>GPGSMTTPNFELYGYFRSSCSGRLRIAFHLKSIPYTRHPVNLLKGEQHSDTYKSLNPTNTVPLLVVSNINNTVSPSSASFSIGQSLAALEYLEEALPTNARPLLPPISNPVARAHVRTICNIIACDVQPVTNLKIQKKVKALDGDPTVWSRDLATQGFGAVEKLLELSAGRFCVGDEITLADVCLVPAVWAAERVGMDLARFPITKRVFEEMLKEEAVQKAHWQKQEDTPEDLRA[4x]

Crystal structures are presented for a putative uncharacterized protein that shares sequence similarity with ζ-class glutathione S-transferases (GSTs) in both apo and glutathione-bound forms. Each protomer consists of an N-­terminal βαβαββα thioredoxin-like fold common to all GSTs as well as a C-­terminal α-helical domain. Based on sequence homology, structural similarity, half-site glutathione binding and sulfate ion H-site binding, the protein investigated here is likely to be a ζ-class GST/MAAI. Glutathione S-transferases (GSTs) are detoxifying enzymes that appear across a wide range of aerobic organisms, including bacteria, fungi, plants and mammals.

The 2.2 Å resolution apo structure contains two pseudosymmetrically related dimers in the asymmetric unit. The apo structure reveals a nonsymmetric homodimer with each protomer comprising two subdomains: a C-terminal helical domain and an N-terminal thioredoxin-like domain that is common to all GSTs. The C. immitis protein exhibits a nonsymmetrical dimer in which one protomer has several more ordered residues than the other; residues 39–52 are dis­ordered in the second protomer. These residues correspond to the cap of the active site and coordinate glutathione in the G-site (see below). All four chains in the asymmetric unit contain a sulfate molecule that binds to the backbone N atom and side-chain hydroxyl of Ser15 as well as the side chain of Gln124 and forms water-mediated interactions with several additional residues. A sulfate ion is observed in approximately the same orientation off Ser15 as in the H-site of the human ζ-class GST crystal structure and is believed to simulate the expected binding of the substrate dichloro­acetic acid. The equivalent Arg190 in the C. immitis structure resides in a different rotomer conformation without forming interactions with the sulfate ion (which is approximately 4.8 Å away in each protomer); it is involved in salt-bridge interactions within the crystal lattice.>[2x]MATDLIMTILPGMTVKVTNPND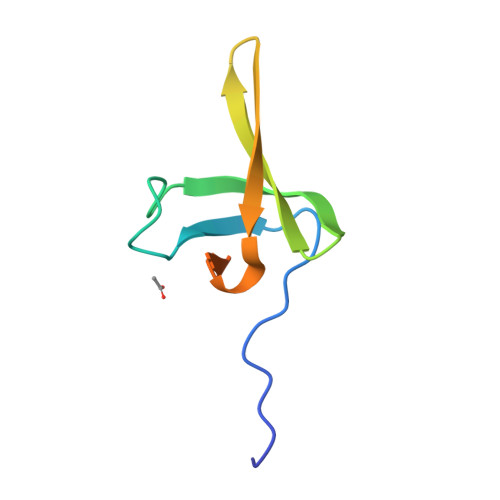TYYQFQGIVQRITDGKVAVLFEGGNWDKLVTFQASELEPVVVTPKEKAKAKK>GATGSVGGGKGSGVGISTGGWVGGSYFTDSYVITKNTRQFLVKIQNDHKYRTENIIPSNAGGKSQRCVSTPWSYFNFNQYSSHFSPQDWQRLTNEYKRFKPRKMHVKIYNLQIKQILSNGADTTYNNDLTAGVHIFCDGEHAYPNATHPWDEDVMPELPYETWYLFQYGYIPVIHELAEMEDANAVEKAIALQIPFFMLENSDHEVLRTGESTEFTFDFDCEWINNERAYIPPGLMFNPKVPTRRAQYIRQHGNTASSNTRIQPYAKPTSWMTGPGLLSAQRVGPAGSDTASWMVVVNPDGTAVNSGMAGVGSGFDPPSGSLRPTDLEYKIQWYQTPEGTNSDGNIISNPPLSMLRDQALYRGNQTTYNLCSDVWMFPNQIWDRYPITRENPIWCKKPRSDKNTIIDPFDGTLAMDHPPGTIFIKMAKIPVPSNNNADSYLNIYCTGQVSCEIVWEVERYATKNWRPERRHTALGLGIGGEENINPTYHVDKNGKYIQPTTWDMCYPIKTN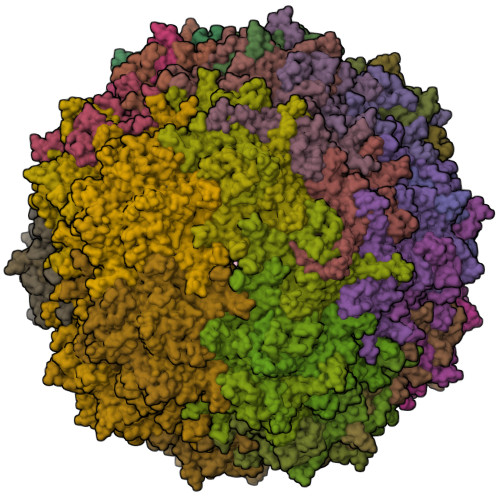INKVL[60x]>TYCVAMRLSSGLAFASDSRTNAGVDHISTFRKLHLFQQPGERTLVVQSAGNLATTQSIVSLLQRRCLDPEQTNLMNVASMYEAATLLGETVREVINRDSGAQQNSHGTDFNCNLLLGGQIKGEGLRLFHIYPQGNFIEATQDTPYFQIGESKYGKPIIDRVLSYDTPLDQAMQCALISMDSTLRSNLSVGLPLDVMIYPLDSFSTEQQYRITEDHPYFMMIRKGWGEGLVSIFAQLPGLKLGRLEHHHHHH[28x]

Anbu shares distant sequence similarity with 20S proteasomes and even more distant similarity with HslV. The threonine, lysine and aspartate residues that form the catalytic triad in HslV and 20S proteasomes are conserved in Anbu. Based on the scattered phylogenetic distribution of Anbu with occurrences in cyanobacteria and proteobacteria, it has been suggested that Anbu may represent an ancestral form of the 20S proteasome or HslV. Anbu predominantly occurs in an operon of four genes in conserved order.

A YbAnbu V14A/G107H variant was more stable and was therefore used in all experiments. YbAnbu exhibits the β-sandwich fold with a characteristic four-layered architecture. In Anbu, the C-terminal helix is much longer than in 20S proteasomes and appears to play a major role in multimer assembly, as it mediates intersubunit contacts in the particle. All three residues are conserved in YbAnbu (T1, D17 and K32). The (putative) S1 pocket is smaller in YbAnbu than in HslV and 20S proteasome subunits due to altered amino acid composition, and other conformations of the β-hairpin region (residues 17–31) and (putative) catalytic lysine residue (K32). In YbAnbu, the hairpin connecting the β2 and β3 strands (residues 17–31) would collide with the P2 and P3 residues in “canonical” position. The basic building block of the YbAnbu particle appears to be a protomer built from two subunits tightly bound to each other, in part by interactions between the Anbu specific C-terminal helices. The YbAnbu protomers are then further assembled into a left-handed helical staircase. Instead, 7 protomers or 14 subunits assemble into a twofold symmetric lock-washer shaped particle. The YbAnbu structure reported in this work differs from all other helical assemblies observed for Anbu by its much smaller rise.>[4x]GSGGGMFGAFVSHRLWSDSGCTTTCITNSIANYVAFGEQIGFPFKSAQVFIAGPRKAVINIQEDDKVELLKMIVKHNLWVVAHGTYLDVPWSRRSAFVTHFIQQELLICKEVGIKGLVLHLGAVEPELIVEGLKKIKPVEGVVIYLETPHNKHHTYKYSTMEQIKELFLRIRNTRLKQIGLCIDTAHIWSSGVNISSYNDAGQWLRSLEN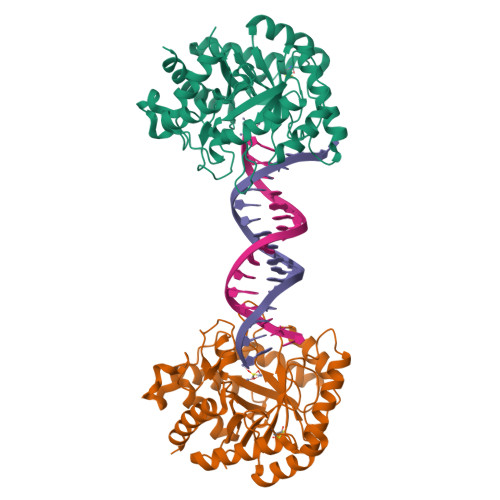IHSVIPPSHIMFHLNDAATECGSGIDRHASLFEGMIWKSYSHKIKQSGLYCFVEYITRHQCPAILERNLGSSMQLQTALTAEFTTLKSLLK>PDARSDARDLTAFQKNILTVLGEEARYGLAIKRELEEYYGEEVNHGRLYPNLDDLVNKGLVEKSELDKRTNEYALTNEGFDAVVDDLEWTLSKFVA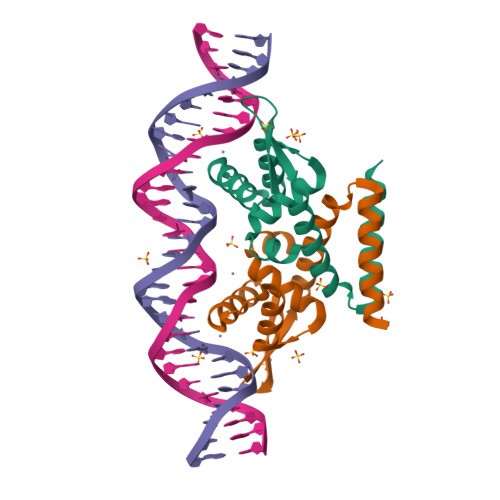DADRRERVETIVADDAAALE[4x]>[4x]TRDQNGTWEME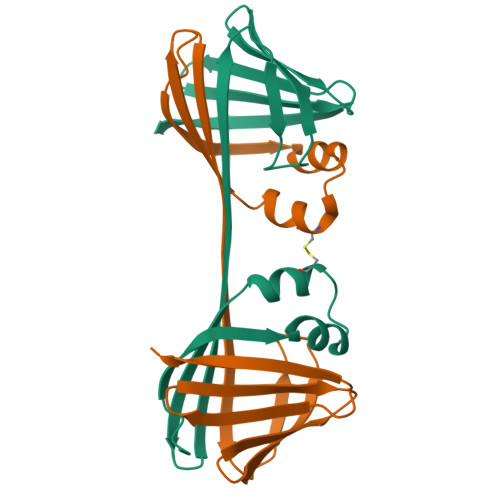SNENFEGYMKALDIDFCTRKIAVRCTQTKVIDQDGDNFKDKTTSTFWWWRNYDVDFTVGVEFDEYTKSLDNRHVKALVTWEGDVLVCVQKGEKENRGWKKWIEGDKLYLELTCGDQVCRQVFKKK> AHMTNGWVIGVDPDIGGAIAVLSPDGSSQVFDNPFVHIVVSEVIRKRLDTKSIIELLRGLDAPPGTTAYIEKSSPFPTDGKQGWWSTGFSYGLWIASLVASGFSVVPVASQTWKAYFGLMRSETPKDDSR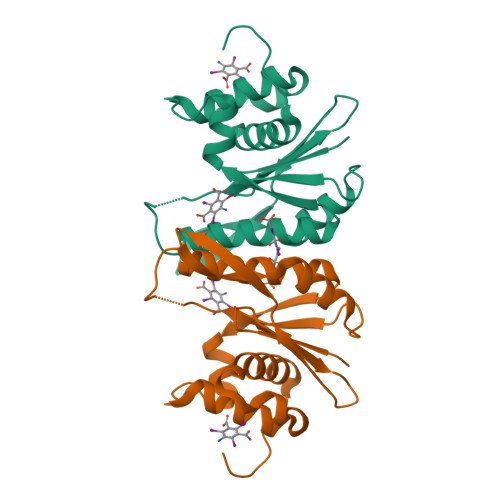QAASILFPDKDQSLKLKKHHGRAEALLLAAYGKGLVLPSGKFSKTSV> MARRYDSRTTTFSPEGRLYQVEYALEAINNASITIGLITKDGVILGADKVFISKLIDKANNYEKIYKIDKHIFCGVAGLNADANILINQSRLYAQRYLYNYNEV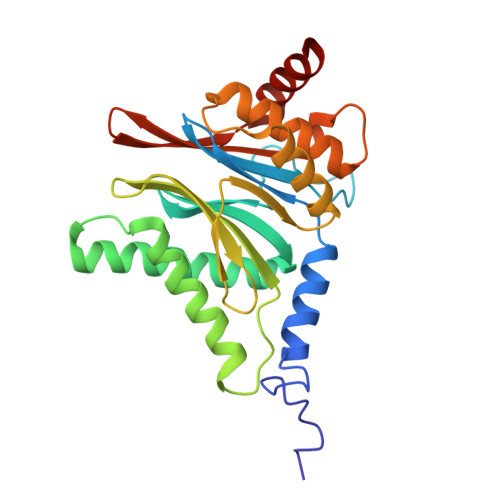QPVSQLVVQICDIKQSYTQYGGLRPYGVSFLIGGYDTKDGYQLYHTDPSGNYSGWFATAIGTNNLTASSVLKQEWKNDMTLEEGLLLALKTLAKSTDTEIPKSEKIELAYLTNKDGEVYQKYLTEKEIEELIKLYTQK> MSHLAELVASAKAAISQASDVAALDNVRVEYLGKKGHLTLQMTTLRELPPEERPAAGAVINEAKEQVQQALNARKAELESAALNARLAAETIDVSLPGRRIENGGLHPVTRTIDRIESFFGELGFTVATGPEIEDDYHNFDALNIPGHHPARADHDTFWFDTTRLLRTQTSGVQIRTMKAQQPPIRIIAPGRVYRNDYDQTHTPMFHQMEGLIVDTNISFTNLKGTLHDFLRNFFEEDLQIRFRPSYFPFTEPSAEVDVMGKNGKWLEVLGCGMVHPNVLRNVGIDPEVYSGFAFGMGMERLTMLRYGVTDLRSF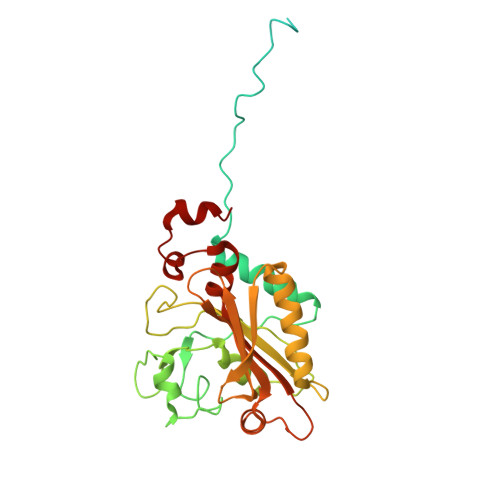FENDLRFLKQFK> MFDNLTDRLSRTLRNISGRGRLTEDNVKDTLREVRMALLEADVALPVVREFINRVKEKAVGHEVNKSLTPGQEFVKIVRNELVAAMGEENQTLNLAAQPPAVVLMAGLQGAGKTTSVGKLGKFLREKHKKKVL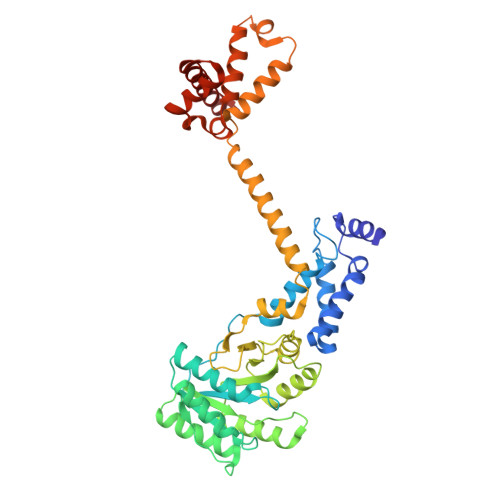VVSADVYRPAAIKQLETLAEQVGVDFFPSDVGQKPVDIVNAALKEAKLKFYDVLLVDTAGRLHVDEAMMDEIKQVHASINPVETLFVVDAMTGQDAANTAKAFNEALPLTGVVLTKVDGDARGGAALSIRHITGKPIKFLGVGEKTEALEPFHPDRIASRILGMGDVLSLIEDIESKVDRAQAEKLASKLKKGDGFDLNDFLEQLRQMKNMGGMASLMGKLPGMGQIPDNVKSQMDDKVLVRMEAIINSMTMKERAKPEIIKGSRKRRIAAGSGMQVQDVNRLLKQFDDMQRMMKKMKKG> HMERPESELIRQSWRVVSRSPLEHGTVLFARLFALEPSLLPLFQGGGQFSSPEDSLSSPEFLDHIRKVMLVIDAAVTNVEDLSSLEEYLTSLGRKHRAVGVRLSSFSTVGESLLYMLEKSLGPDFTPATRTAWSRLYGAVVQAMSRGWDG

Ngb is over-expressed in hypoxic conditions and it may be involved in gas/redox sensing, radical scavenging, and/or signal transduction. Notably, hexacoordination in Ngb accounts for a peculiar structural rearrangement and complex kinetics upon ligand binding, which takes place when the distal histidine (His(E7)64), engaged in internal iron hexacoordination, dissociates from the heme. The dissociation of His64 is the rate-limiting step for ligand binding and it triggers a repositioning of the heme which slides further inside a large internal cavity. In this study, we spectroscopically and structurally characterized three Ngb mutants aiming at pinpointing key features: a CD loop mutant with enhanced flexibility (Gly-loop), the F106A mutant and the double Gly-loop/F106A mutant.

Crystals of the Gly-loop mutant tend to dissolve upon exposure to CO in the reduced Fe2+ state. However, by freezing crystals before complete disruption, we managed to determine a structure in which we observed about 40% CO ligation and a concomitant swung out histidine conformation. Moreover electron density appeared for the 49–56 segment that could be successfully built. We propose a sequence of events for ligand binding to neuroglobin, in which after spontaneous rupture of the 6th coordination bond of His64 to the heme iron, exogenous diatomic ligands such as CO can be coordinated by the heme only upon swinging out of His64, having isolated and determined the structure of this intermediate in the Gly-loop mutant where the Tyr44-propionate barrier is absent. The mobilization of the CD-loop-D-helix unit could facilitate the His64 dissociation from the heme iron, unlocking its swing-out displacement, thus leading to the increased CO binding velocities observed by rapid mixing. Removal of the barrier to His64 early swinging out increases the velocity of binding by one order of magnitude, reaching a much faster rate limiting step in the Gly-loop mutant with respect to WT Ngb.>GAMGMNGQGATSIPGEVAEQAMHWHLE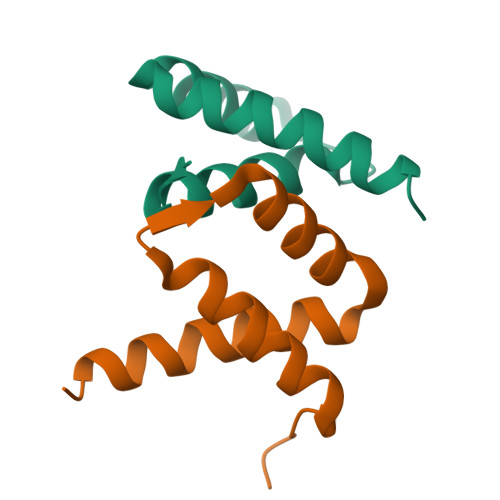LQEPAVSAATLAACMSWRQAHPLHEHAWQRTQVFAQRLREMRSPGQRPLAHAALRPQQS[4x]> MSVTIDHTTENAAPAQAPVSDRAWALFRALDGKGLVPDGYVEGWKKTFEEDFSPRRGAELVARAWTDPEFRQLLLTDGTAAVAQYGYLGPQGEYIVAVEDTPTLKNVIVCSLCACTAWPILGLPPTWYKSFEYRARVVREPRKVLSEMGTEIASDIEIRVYDTTAETRYMVLPQRPAGTEGWSQEQLQEIVTKDCLIGVAIPQVPTV;> MDGVHDLAGVQGFGKVPHTVNADIGPTFHAEWEHLPYSLMFAGVAELGAFSVDEVRYVVERMEPRHYMMTPYYERYVIGVATLMVEKGILTQDELESLAGGPFPLSRPSESEGRPAPVETTTFEVGQRVRVRDEYVPGHIRMPAYCRGRVGTISHRTTEKWPFPDAIGHGRNDAGEEPTYHVKFAAEELFGSDTDGG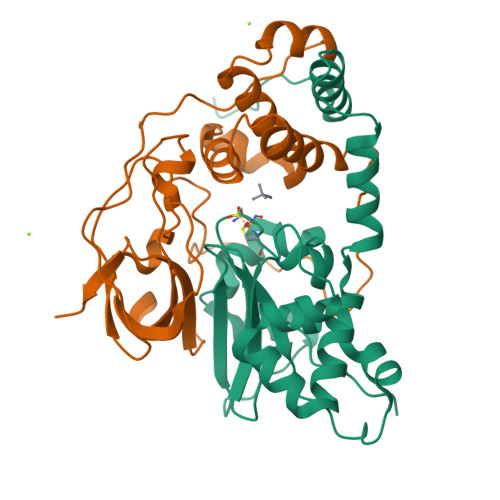SVVVDLFEGYLEPAA>[4x]MRGSHHHHHHGSDQVSLGVVGIGKIARDQHLPAIDAEPGFKLTACASRHAEVTGVRN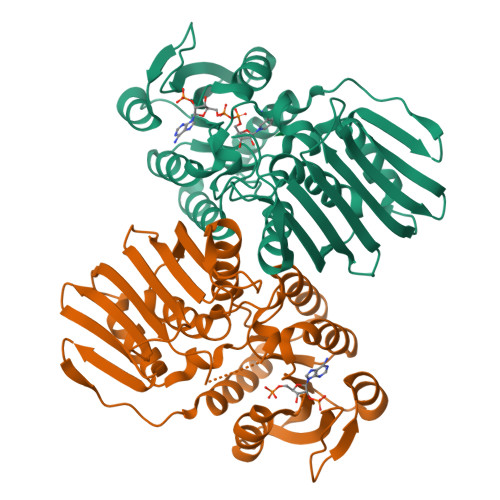YRDLRALLAAERELDAVSLCAPPQVRYAQARAALEAGKHVMLEKPPGATLGEVAVLEALARERGLTLFATWHSRCASAVEPAREWLATRAIRAVQVRWKADVRRWHPGQQWIWEPGGLGVFDPGINALSIVTRILPRELVLREATLIVPSDVQTPIAAELDCADTDGVPVRAEFDWRHGPVEQWEIAVDTADGVLAISRGGAQLSIAGEPVELGPEREYPALYAHFHALIARGESDVDVRPLRLVADAFLFGRRVQTDAFGR> AVGPVADLTITDAAVSPDGFSRQAVVVNGVTPGPLVAGNIGDRFQLNVIDNLTNHTMLKSTSIHWHGFFQHGTNWADGPAFINQCPISPGHSFLYDFQVPDQAGTFWYHSHLSTQYCDGLRGPFVVYDP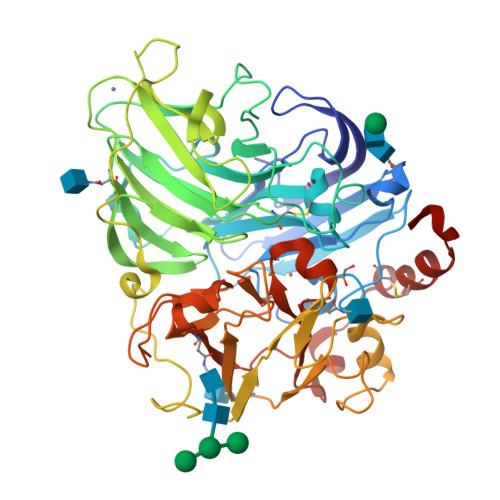NDPHASRYDVDNDDTVITLADWYHTAAKLGPRFPLGADATLINGKGRAPSDTTAELSVIKVTKGKRYRFRLVSLSCDPNHTFSIDGHNLTIIEVDSVNSQPLEVDSIQIFAAQRYSFVLDANQAVDNYWIRANPNFGNVGFDGGINSAILRYDGAPAVEPTTNQTTSVKPLNEVDLHPLVSTPVPGSPSSGGVDKAINMAFNFNGSNFFINGASFVPPTVPVLLQILSGAQTAQDLLPSGSVYVLPSNASIEISFPATAAAPGAPHPFHLHGHTFAVVRSAGSTVYNYDNPIFRDVVSTGTPAAGDNVTIRFDTNNPGPWFLHCHIDFHLEGGFAVVMAEDTPDVKAVNPVPQAWSDLCPTYDALDPNDQ> MMRFAIAAALGALLAVAAAPAAVAAARRPPWDIARFRPALRVAKLQAPDSVQRKDVRSFPNFQADHFYSENRDMVFVMGGDSQRSELRFLDEWSVRTSSTRRMVGVLTLPTPLRGMKHFTWMQVAGGSKGKKPLLRLSWHDKREQGGKDLRNTMLATVRLNNKSGDAGRFKKIVLGTRPSGRFVADVRVERSRLTVRLNGRKLVDEDVGYWTYSTNYFKAGVYVQEGSPDARVVFHGLTVS

In heterotrophic bacteria that use alginates as crucial nutrients, alginate lyases depolymerize alginate into alginate oligosaccharides (AOSs) and then into monomers for assimilation into the central metabolism. The overall structures of these PL7 alginate lyases are similar, showing a β-jelly roll fold composed of two antiparallel β-sheets with a deep cleft. The noteworthy structural differences among the solved PL7 structures are the loops around the deep cleft, which are variable in length and sequence and involved in alginate substrate binding with the deep cleft. Structural study on several PL7 alginate lyases reveals that two loops around the substrate binding cleft determine product distribution.

Similar to AlyV, several PyAly mutants and two oligomeric substrates (M8 and M5) were used to determine the structures of PyAly-oligosaccharide complexes. The structures of the PyAlyH125A-M8 complex and the PyAlyH125A_Y223A-M5 complex were solved at 1.62 Å and 1.70 Å, respectively. Except for the sugar units bound at subsites −3, −2, and −1, the other sugar units of M8 were not observed in the structure of the PyAlyH125A-M8 complex, which was similar to the observation in the structure of the AlyVR91A-M8 complex. -3 subsite: The side chain of Arg143 formed two hydrogen bonds with the C-5 carboxyl group. -2 subsite: The side chain of Lys172 formed hydrogen bonds with the hydroxyl groups at the C-2 and C-3 positions. -1 subsite: The side chain of Arg159 formed two hydrogen bonds with the C-5 carboxyl group. At subsite -1, the three-dimensional position of the sugar unit in the AlyVR91A-M8 complex resembled that in the PyAlyH125A-M8 complex. However, a clear angle was observed between the two sugar units at subsite -2; that is, the directions of the two C-5 carboxyl groups at subsite -2 were different. For PyAly, loop1 consists of residues Thr108 to Lys117, and loop2 consists of residues Arg159 to Phe170. More interestingly, Lys131 from AlyV loop1 formed hydrophobic contacts with the sugar unit at subsite -2, whereas PyAly loop1 was too short to form any interactions with the sugar unit at this subsite.>[2x]MQIPLCANL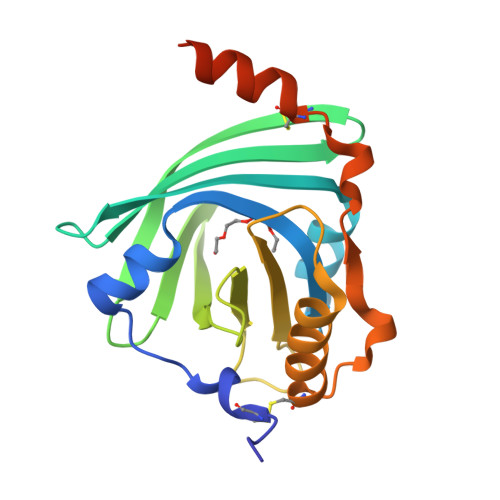VPVPITNATLDRITGKWFYIASAFRNEEYNKSVQEIQATFFYFTPNKTEDTIFLREYQTRQNQCFYNSSYLNVQRENGTVSRYEGGREHVAHLLFLRDTKTLMFGSYLDDEKNWGLSFYADKPETTKEQLGEFYEALDCLRIPRSDVMYTDWKKDKCEPLEKQHEKERKQEEGESHHHHHH>[2x]VADRYAVYWNSSNPRFQRGDYHIDVCINDYLDVFCPHYEDSVPEDKTERYVLYMVNFDGYSACDHTSKGFKRWECNRPHSPNGPLKFSEKFQLFTPFSL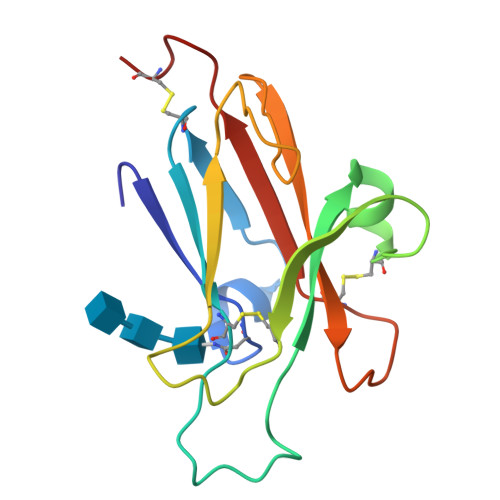GFEFRPGREYFYISSAIPDNGRRSCLKLKVFVRPTNSCM> MGSDKIHHHHHHENLYFQGMTATELVNAYYAAFNAGDMPAFLALLSEDVIHDINQGERQMGKARFAAFMEKMNRCYRERLADIVVMQNADGSRAAAEFTVHGQYLADDEGLPTANGQTYVLPAGAFFYIHCGKIARVT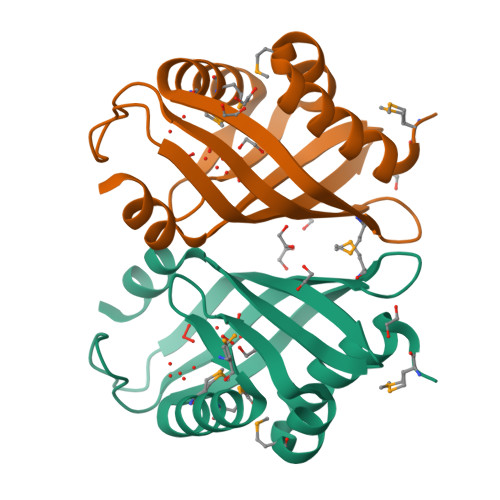NYYNLNDWVEQVA> GPGSMDSGRFDTAVYARRLAAAAAATEQAGLAGLVITPGYDLRYLIGSRADTFERLTALVLPASGVPTIVLPRLELASLKESAASDLGVCVRDWVDGDDPYQLVAVALGGAPAATAVTDSMPALHLLPLADALGVLPVLATDVLRQLRMVKEAAEVDALAKAGAAIDRVHARVPAFLVPGRTEAQVAADIAEAIVAEGHSAVAFVIVGSGPHGADPHHGYSDRKLQVGDIVVVDIGGTYEPGYYSDSTRTYSIGDPSPDVAQQYSALQRAQRAAVDAVRPGVTAAQVDAAARDVLADAGLAEYFVHRTG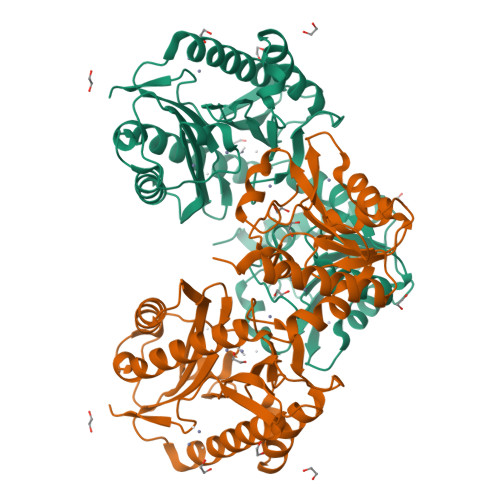HGIGLCVHEEPYIVAGNELPLVAGMAFSIEPGIYFPGRWGARIEDIVVVTENGALSVNNRPHELMVVPV> SAVQQLQPTQAGISMAPSAQGAMVRIRNPAVSSSRGGITVLTHSELSAEIGVTDSIVVSSELVMPYTVGTWLRGVAANWSKYSWLSVRYTYIPSCPSSTAGSIHMGFQYDMADTVPVSVNQLSNLRGYVSGQVWSGSAGLCFINGTRCSDTSTAISTTLDVSKLGKKWYPYKTSADYATAVGVDVNIATPLVPARLVIALLDGSSSTA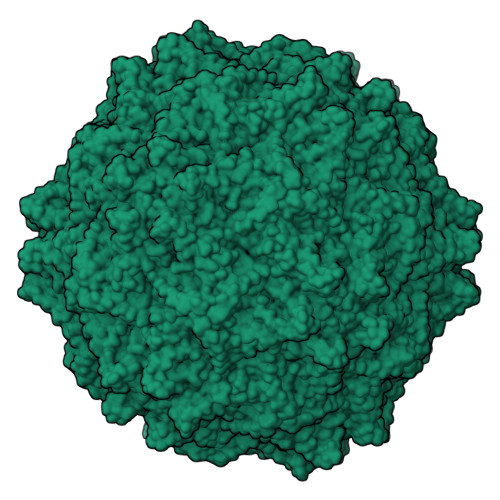VAAGRIYCTYTIQMIEPTASALNN>MEFSIDLNNLIGIIAGAITTSALIPQALKIYKTKSARDVSLAMFIFMAIGITLWFFYGVLIKEIP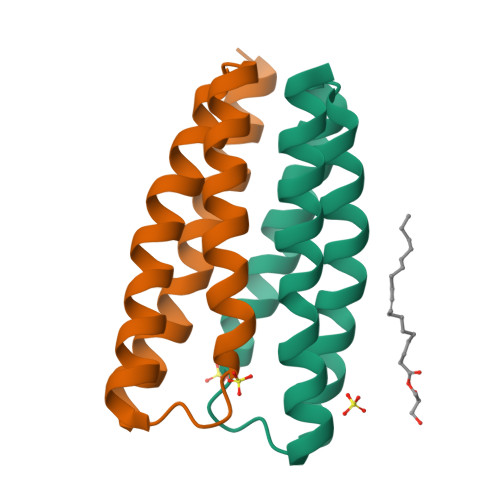VILANLISLILIFLIIFMKIRYGHHHHHH[6x]>ALRGTVTDFSGFDGEADAEVLEKAMEGLGTDEDSILNLLTARSNAQRQQIAEEFETLFGRDLVNDMKSELTGKFEKLIVALMKPSRLYDAYELKHALKGAGTDEKVLTEIIASRTPEELRAIKQAYEEEYGSNLEDDVVGDTSGYYQRMLVVLLQANRDPDTAIDDAQVELDAQALFQAGELKWGTDEEEFITILGTRSVSHLRRVFDKYMTISGFQIEETIDRETSGNLENLLLAVVKSIRSIPAYLAETLYYAMKG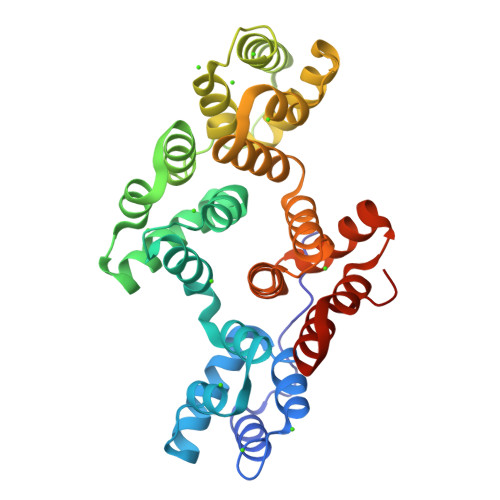AGTDDHTLIRVIVSRSEIDLFNIRKEFRKNFATSLYSMIKGDTSGDYKKALLLLSGGEDD[2x]MGME1 (also known as DDK1) is a highly conserved, mitochondria-specific DNase. Human MGME1 (HsMGME1) protein is composed of 344 amino acids and belongs to the PD-(D/E)XK nuclease superfamily. However, in contrast to DNA2 (2–5) and many other mitochondrial DNases, MGME1 can cleave various types of DNA substrates with a preference for single-stranded DNAs (ssDNA). Structural analysis and comparison suggest that MGME1 follows a two-cation-assisted catalytic mechanism of substrate cleavage.

To test our hypothesis, we constructed one HsMGME1 mutant with His180 substituted by Gln180, which is similar to His180 in size but neutral in charge. Using this H180Q mutant, we successfully solved one HsMGME1 ternary complex structure, H180Q–ssDNA2–Ca2+. One six-coordinated Ca2+ ion was bound at the active site of HsMGME1. The Ca2+ ion coordinates with the O atom of acetic acid (ACT), the side chain OD2 atom of Asp238, the side chain OD1 atom of Asp251, the main chain O atom of Trp252, as well as two water molecules. Beside Ca2+-coordination, water molecule W1 also forms one H-bond (2.6 Å) with the side chain NZ atom of Lys253. The residue Gln180 does not coordinate Ca2+; compared with His180 in the HsMGME1–Mn2+ structure, the side chain of Gln180 is rotated clockwise around the CA-CB bond for about 150° in the H180Q-ssDNA2-Ca2+ complex. Though they are not identical in coordination, the orientations of the Ca2+ and the A-site Mn2+ are very similar in the H180Q-ssDNA2-Ca2+ and HsMGME1–Mn2+ structures. As indicated by the very low root mean square deviation value (rmsd, 0.7 Å), the overall structure of H180Q–ssDNA2–Ca2+ is very similar to that of the HsMGME1–ssDNA2 complex. Instead of forming an H-bond interaction, the NZ atom of Lys253 in the HsMGME1-ssDNA2 structure almost overlaps with the Ca2+-coordinating water molecule W1 of the H180Q–ssDNA2–Ca2+ complex. Though one Ca2+ ion was bound at the A-binding site, the B-binding site was not occupied by any cations in the H180Q–ssDNA2–Ca2+ complex, which may have weakened the overall DNA coordinating ability of Ca2+ and led to the shifting of the A5 nucleotide.

> GEDRRVPQNWFPIFNPERSDKPNASDPSVPLKIPLQRNVIPSVTRVLQQTMTKQQVFLLERWKQRMILELGEDGFKEYTSNVFLQGKRFQEALESILSPQETLKERDENLLKSGYIESVQHILKDVSGVRALESAVQHETLNYIGLLDCVAEYQGKLCVIDWKTSEKPKPFIQSTFDNPLQVVAYMGAMNHDTNYSFQVQCGLIVVAYKDGSPAHPHFMDAELCSQYWTKWLLRLEEYTEKKKNQNIQKPEYSE>MNPYERGPNPTDALLEARSGPFSVSEENVSRLSASGFGGGTIYYPRENNTYGAVAISPGYTGTEASIAWLGERIASHGFVVITIDTITTLDQPDSRAEQLNAALNHMINRASSTVRSRIDSSRLAVMGHAMGGGGSLRLASQRPDLKAAIPLTPWHLNKNWSSVTVPTLIIGADLDTIAPVATHAKPFYNSLPSSISKAYLELDGATHFAPNIPNKIIGKYSVAWLKRFVDNDTRYTQFLCPGPRDGLFGEVEEYRSTCPF[4x]

Cutinase is an esterase that belongs to the α/β-hydrolase superfamily and primarily hydrolyzes cutin from plants. Unlike lipases, cutinases lack the active site-covering lid structure such that the substrate-binding cleft is exposed and directly accessible from bulk solution. In addition, the substrate-binding site is more expansive in cutinases compared to esterases, benefiting the binding of bulkier macromolecules. In this work, we investigate the PBAT hydrolysis potency of cutinases and PET-degrading enzymes, and find that cutinases outcompete other reported enzymes.

To better illustrate whether DM strategy alters the substrate-binding mode, we solved crystal structures of an inactive WT TfCut variant (S170A) and its complex with the PBAT analog. The WT TfCut contains the combination of His/Phe in positions of 224 and 228 below W195 and this pair fixes the W195-bareing loop and its indole ring in the C-type conformation. This leads to a narrower substrate entering portal (circled in Fig. 4a). The same structural feature should be shared by canonical cutinases as revealed in the LCC-ICCG complex because the His/Phe duo is strictly conserved in similar enzymes.>RALHRR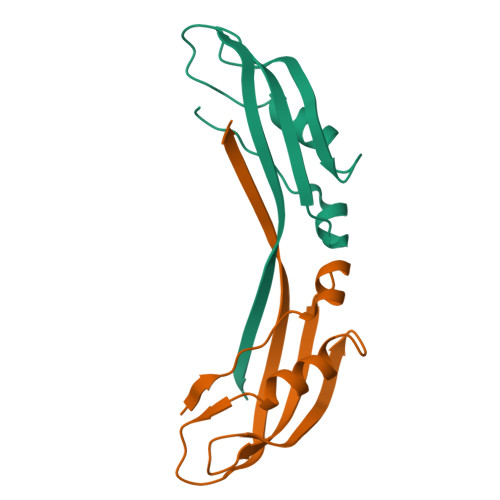VNYPSRAKALGVEGKVRVKFDITGSGTVTNVQVLSETPDGVFGDDVVKDMARWRYRTEAPVENQVVSIVFKLNGHIRVDDQ[2x]>MTISRTQQIQQLEQEWTSPRWKNITRPYSAEDVIKLRGSVNPECTFAQNGAKKLWELLHGGSRKGYINCLGALTGGQALQQAKAGVEAIYMSGWQVAADANTASSMYPDQSLYPVDSVPAVVKRINNSFRRADQIQWSNNIEPGSKGYTDYFLPIVADAEAGFGGVLNAFELMKAMIEAGAAGVHFEDQLAAVKKCGHMGGKVLVPTQEAIQKLVAARLAADVLGVPTLLIARTDADAADLLTSDCDPYDREFITGDRTAEGFFRTRAGIEQAISRGLAYAPYADLVWCETSTPDLALAKRFADAVHAQFPGKLLAYNCSPSFNWKKNLTDQQIASFQDELSAMGYKYQFITLAGIHSMWFNMFDLAHAYAQGEGMKHYVEKVQQPEFAS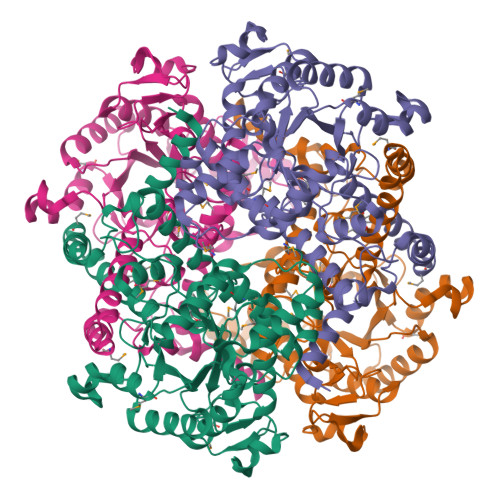VDRGYTFASHQQEVGTGYFDKVTNIIQGGASSVTALTGSTEEQQF[2x]[(2~{S},3~{S},5~{S},6~{S},8~{S},9~{S},10~{R},13~{R},14~{R},17~{R})-17-[(2~{R})-6,6-dimethylheptan-2-yl]-10,13-dimethyl-2,3-disulfooxy-2,3,4,5,6,7,8,9,11,12,14,15,16,17-tetradecahydro-1~{H}-cyclopenta[a]phenanthren-6-yl] 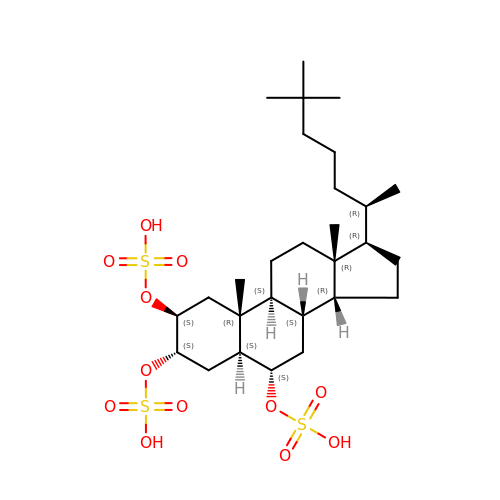hydrogen sulfate | C28 H50 O12 S3 | MNVNGGMQJFYHMK-NZLCMVQPSA-N> EKIKICLQKQVNSSFSLHNGFGGNLYATEEKRMFELVKPKAGASVLNQSTWIGFGDSRTDKSNSAFPRSADVSAKTADKFRFLSGGSLMLSMFGPPGKVDYLYQGCGKHKVFYEGVNWSPHAAINCYRKNWTDIKLNFQKNIYELASQSHCMSLVNALDKTIPLQVTAGTAGNCNNSFLKNPALYTQEVKPSENKCGKENLAFFTLPTQFGTYECKLHL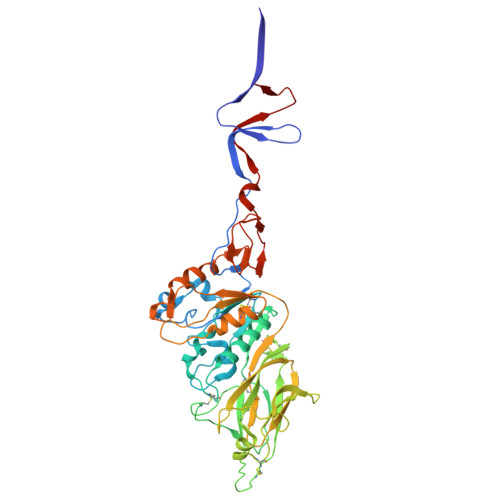VASCYFIYDSKEVYNKRGCDNYFQVIYDSFGKVVGGLDNRVSPYTGNSGDTPTMQCDMLQLKPGRYSVRSSPRFLLMPERSYCFDMKEKGPVTAVQSIWGKGRESDYAVDQACLSTPGCMLIQKQKPYIGEADDHHGDQEMRELLSGLDYEARCISQSGWVNETSPFTEKYLLPPKFGRCPLAAKEESIPKIPDGLLIPTSGTDTTVTKPKSR> MNTKYNKEFLLYLAGFVDADGSIIAQIAPNQSSKFKHRLKLTFQVTQKTQRRWFLDKLVDEIGVGYVRGSGSVSNYILSEIKPLHNFLTQLQPFLKLKQKQANLVLKIIEQLPSAKESPDKFLEVCTWVDQIAALNDSKTRKTTSETVRAV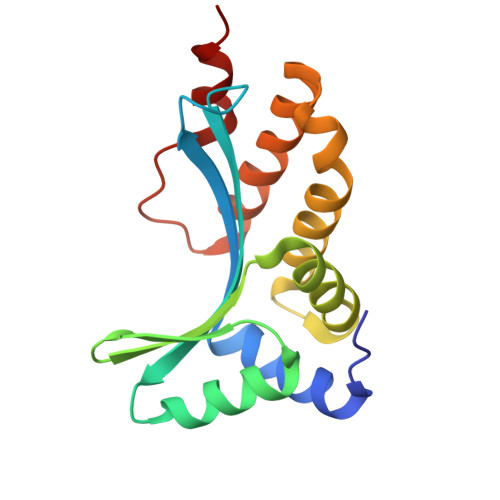LD> GANHFHVFVGDLSPEITTEDIKAAFAPFGRISDARVVKDMATGKSKGYGFVSFFNKWDAENAIQQMGGQWLGGR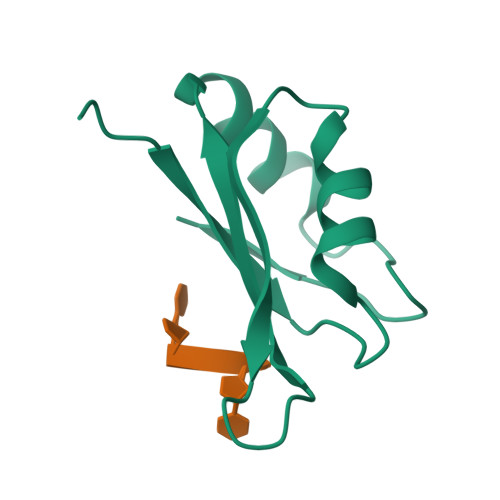QIRTNW>MATQGVFTLPANTRFGVTAFANSSNTQTVNVLVNNETAATFSGQSTNNAVIGTQVLNSGSSGKVQVQVSVNGRPSDLVSAQVILTNELNFALVGSEDGTDND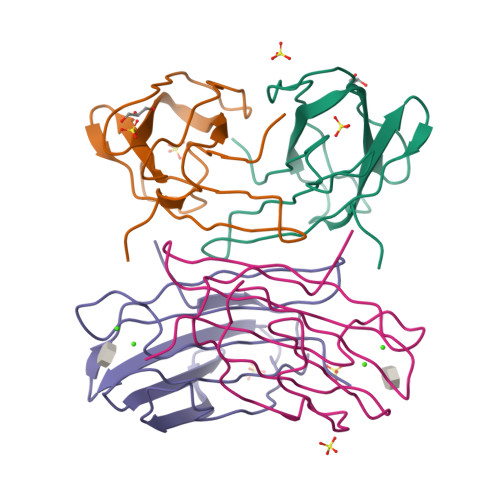YNDAVVVINWPLG[4x]>[4x]MGMWASLDALWEMPAEKRIFGAVLLFSWTVYLWETFLAQRQRRIYKTTTHVPPELGQIMDSETFEKSRLYQLDKSTFSFWSGLYSETEGTLILLFGGIPYLWRLSGRFCGY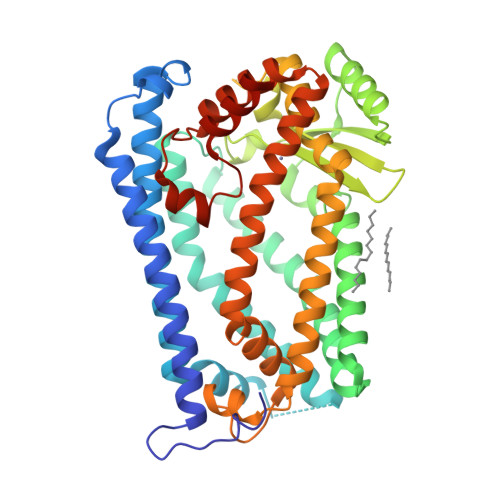AGFGPEYEITQSLVFLLLATLFSALAGLPWSLYNTFVIEEKHGFNQQTLGFFMKDAIKKFVVTQCILLPVSSLLLYIIKIGGDYFFIYAWLFTLVVSLVLVTIYADYIAPLFDKFTPLPEGKLKEEIEVMAKSIDFPLTKVYVVEGSKRSSHSNAYFYGFFKNKRIVLFDTLLEEYSVLNKDIQEDSGMEPRNEEEGNSEEIKAKVKNKKQGCKNEEVLAVLGHELGHWKLGHTVKNIIISQMNSFLCFFLFAVLIGRKELFAAFGFYDSQPTLIGLLIIFQFIFSPYNEVLSFCLTVLSRRFEFQADAFAKKLGKAKDLYSALIKLNKDNLGFPVSDWLFSMWHYSHPPLLERLQALKTMKQHAENLYFQ>[4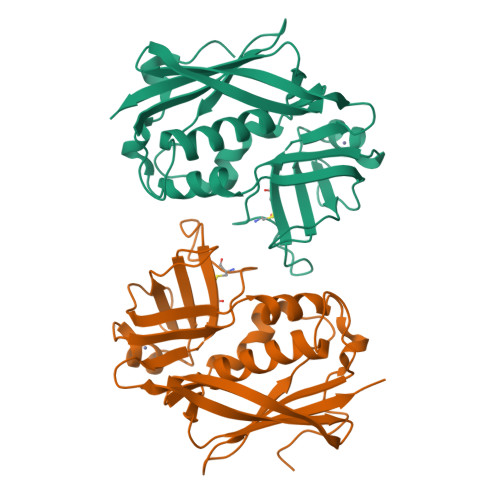x]QQDPDPSQLHRSSLVKNLQNIYFLYEGDPVTHENVKSVDQLLSHDLIYNVSGPNYDKLKTELKNQEMATLFKDKNVDIYGVEYYHLCYLCENAERSACIYGGVTNHEGNHLEIPKKIVVKVSIDGIQSLSFDIETNKKMVTAQELDYKVRKYLTDNKQLYTNGPSKYETGYIKFIPKNKESFWFDFFPEPEFTQSKYLMIYKDNETLDSNTSQIEVYLTTK> MKKEKIDLFYGALLADIGKVIQRATGERKKHALVGADWFDEIADNQVISDQIRYHMANYQSDKLGNDHLAYITYIADNIASGVDRRQSNEESDEDTSAKIWDTYTNQADIFNVFGAQTDKRYFKPTVLNLKSKPNFASATYEPFSKGDYAAIATRIKNELAEFEFNQVQIDSLLNLFEATLSFVPSSTNTKEIADISLADHSRLTAAFALAIYDYLEDKGRHNYKEDLFTKVSAFYEEEAFLLASFDLSGIQDFIYNINIATNGAAKQLKARSLYLDFMSEYIADSLLDKLGLNRANMLYVGGGHAYFVLANTEKTVETLVQFEKDFNQFLLANFQTRLYVAFGWGSFAAKDIMSELNSPESYRQVYQKASRMISKKKISRYDYQTLMLLNRGGKSSERECEICHSVENLVSYHDQKVCDICRGLYQFSKEIAHDHFIITENEGLPIGPNACLKGVAFEKLSQEAFSRVYVKNDYKAGTVKATHVFVGDYQCDEIYNYAALSKNENGLGIKRLAVVRLDVDDLGAAFMAGFSQQGNGQYSTLSRSATFSRSMSLFFKVYINQFASDKKLSIIYAGGDDVFAIGSWQDIIAFTVELRENFIKWTNGKLTLSAGIGLFADK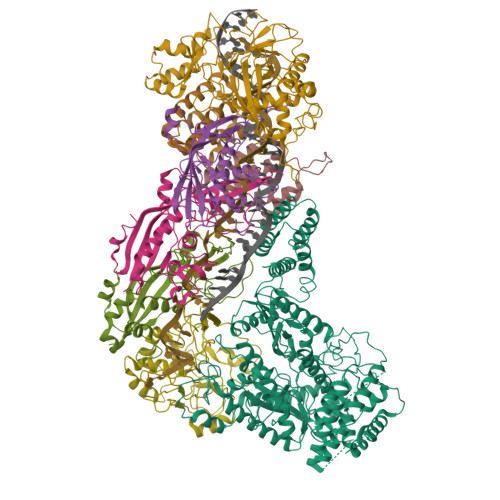TPISLMAHQTGELEEAAKGNEKDSISLFSSDYTFKFDRFITNVYDDKLEQIRYFFNHQDERGKNFIYKLIELLRNHDRMNMARLAYYLTRLEELTRETDRDKFKTFKNLFYSWYTNKNDKDRKEAELALLLYIYEIRKD;>[2x]MTILTDENYVDIAEKAILKLERNTRNRKNPDAFFLTTSKLRNLLSLTSTLFDESKVKEYDALLDRIAYLRVQFVYQAGREIAVKDLIEKAQILEALKEIKDRETLQRFCRYMEALVAYFKFYGGKD;>MTFAKIKFSAQIRLETGLHIGGSDAFAAIGAINSPVIKDPITNLPIIPGSSLKGKMRTLLAKVYNEKVAEKPSDDSDILSRLFGNSKDKRFKMGRLIFRDAFLSNADELDSLGVRSYTEVKFENTIDRITAEANPRQIERAIRNSTFDFELIYEITDENENQVEEDFKVIRDGLKLLELDYLGGSGSRGYGKVAFENLKATTVFGNYDVKTLNELLTAEV[3x];> MTYKLYIMTFQNAHFGSGTLDSSKLTFSADRIFSALVLEALKMGKLDAFLAEANQDKFTLTDAFPFQFGPFLPKPIGYPKHDQIDQSVDVKEVRRQAKLSKKLQFLALENVDDYLNGELFENEEHAVIDTVTKNQPHKDDNLYQVATTRFSNDTSLYVIANESDLLNELMSSLQYSGLGGKRSSGFGRFELDIQNIPLELSDRLTKNHSDKVMSLTTALPVDADLEEAMEDGHYLLTKSSGFAFSHATNENYRKQDLYKFASGSTFSKTFEGQIVDVRPLDFPHAVLNYAKPLFFKLEV;> MKNDYRTFKLSLLTLAPIHIGNGEKYTSREFIYENKKFYFPDMGKFYNKMVEKRLAEKFEAFLIQTRPNARNNRLISFLNDNRIAERSFGGYSISETGLESDKNPNSAGAINEVNKFIRDAFGNPYIPGSSLKGAIRTILMNTTPKWNNENAVNDFGRFPKENKNLIPWGPKKGKEYDDLFNAIRVSDSKPFDNKSLILVQKWDYSAKTNKAKPLPLYRESISPLTKIEFEITTTTDEAGRLIEELGKRAQAFYKDYKAFFLSEFPDDKIQANLQYPIYLGAGSGAWTKTLFKQADGILQRRYSRMKTKMVKKGVLKLTKAPLKTVKIPSGNHSLVKNHESFYEMGKANFMIKEIDK>SHMEAHLYMQVQIVAEDQFCGHQGNDMYDEEKVKYTVFKVLKNSSLAEFVQSLSQTMGFPQDQIRLWPMQARSNGTKRPAMLDNEADGNKTMIELSDNENP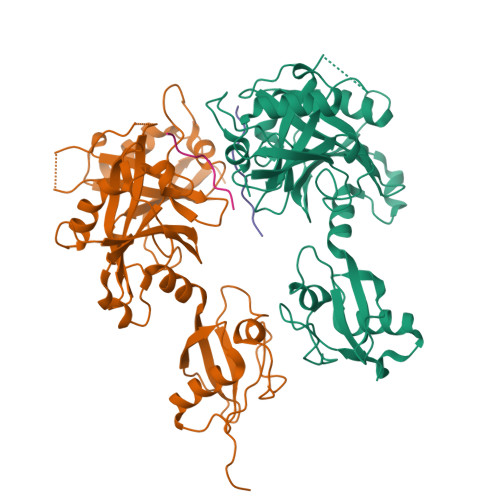WTIFLETVDPELAASGATLPKFDKDHDVMLFLKMYDPKTRSLNYCGHIYTPISCKIRDLLPVMCDRAGFIQDTSLILYEEVKPNLTERIQDYDVSLDKALDELMDGDIIVFQKDDPENDNSELPTAKEYFRDLYHRVDVIFCDKTIPNDPGFVVTLSNRMNYFQVAKTVAQRLNTDPMLLQFFKSQGYRDGPGNPLRHNYEGTLRDLLQFFKPRQPKKLYYQQLKMKITDFEN[4x];>[4x]RGRKRHCKTKHLE>[4x]SKKRQWALEDFEIGRPLGKGKFGNVYLAREKQSKFILALKVLFKAQLEKAGVEHQLRREVEIQSHLRHPNILRLYGYFHDATRVYLILEYAPLGTVYRELQKLSKFDEQRTATYITELANALSYCHSKRVIHRDIKPENLLLGSAGELKIADFGWSVHAPSSRRDTLCGTLDYLPPEMIEGRMHDEKVDLWSLGVLCYEFLVGKPPFEANTYQETYKRISRVEFTFPDF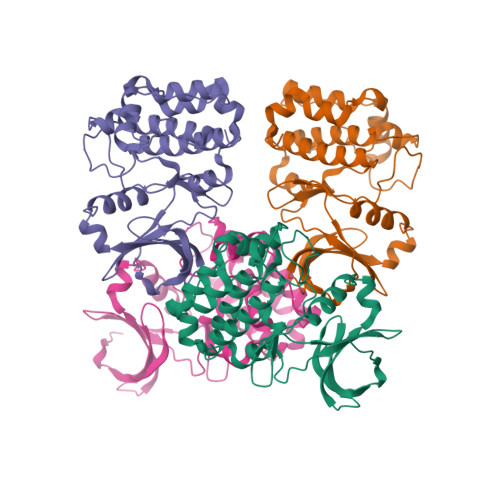VTEGARDLISRLLKHNPSQRPMLREVLEHPWITANSSKPSNCQNKESASK> MAGSPELVVLDPPWDKELAAGTESQALVSATPREDFRVRCTSKRAVTEMLQLCGRFVQKLGDALPEEIREPALRDAQWTFESAVQENISINGQAWQEASDNCFMDSDIKVLEDQFDEIIVDIATKRKQYPRKILECVIKTIKAKQEILKQYHPVVHPLDLKYDPDPAPHMENLKCRGETVAKEISEAMKSLPALIEQGEGFSQVLRMQPVIHLQRIHQEVFSSCHRKPDAKPE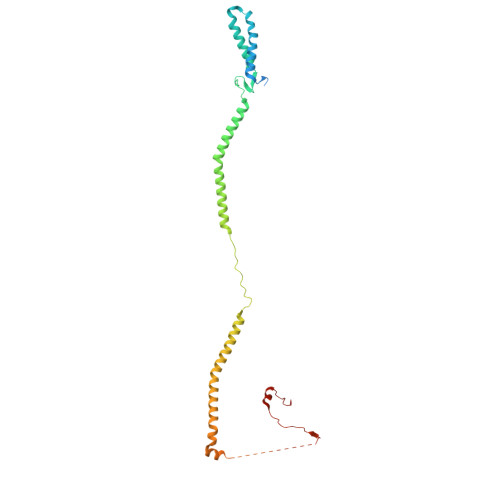NFITQIETTPTETASRKTSDMVLKRKQTKDCPQRKWYPLRPKKINLDT>MRLFLSLPVLVVVLSIVLEGPAPAQGTPDVSSALDKLKEFGNTLEDKARELISRIKQSELSAKMREWFSETFQKVKEKLKIDS[2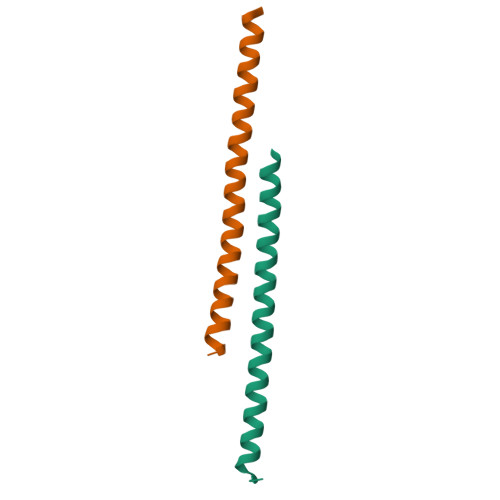x]> MLKLIVKNGYVIDPSQNLEGEFDILVENGKIKKIDKNILVPEAEIIDAKGLIVCPGFIDIHVHLRDPGQTYKEDIESGSRCAVAGGFTTIVCMPNTNPPIDNTTVVNYILQKSKSVGLCRVLPTGTITKGRKGKEIADFYSLKEAGCVAFTDDGSPVMDSSVMRKALELASQLGVPIMDHCEDDKLAYGVINEGEVSAL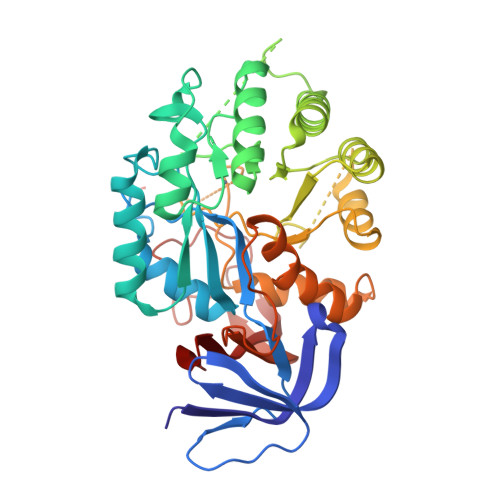LGLSSRAPEAEEIQIARDGILAQRTGGHVHIQHVSTKLSLEIIEFFKEKGVKITCEVNPNHLLFTEREVLNSGANARVNPPLRKKEDRLALIEGVKRGIIDCFATDHAPHQTFEKELVEFAMPGIIGLQTALPSALELYRKGIISLKKLIEMFTINPARIIGVDLGTLKLGSPADITIFDPNKEWILNEETNLSKSRNTPLWGKVLKGKVIYTIKDGKMVYKD> AECSVDIQGNDQMQFNTNAITVDKSCKQFTVNLSHPGNLPKNVMGHNWVLSTAADMQGVVTDGMASGLDKDYLKPDDSRVIAHTKLIGS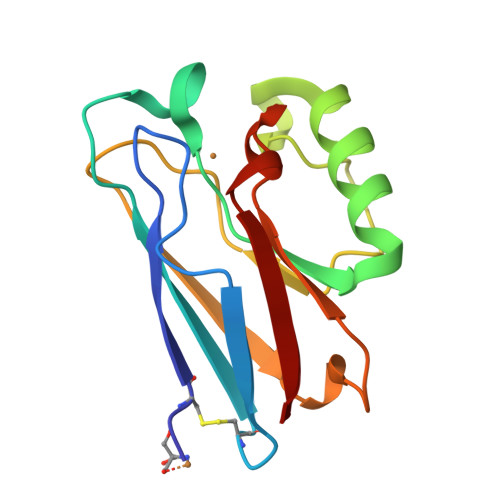GEKDSVTFDVSKLKEGEQYMFFDTFPGHSALEKGTLTLK> FWLP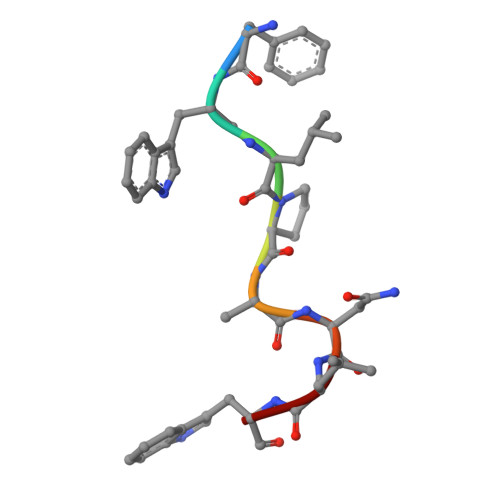ANLW>MNELVDTTEMYLRTIYDLEEEGVTPLRARIAERLDQSGPTVSQTVSRMERDGLLRVAGDRHLELTEKGRALAIAVMRKHRLAERLLVDVIGLPWEEVHAEACRWEHVMSEDVERRLVKVLNNPTTSPFGNPIPGLDELGVGPEPGADDANLVRLTELPAGSPVAVVVRQLTEHVQGDIDLITRLKDAGVVPNARVTVETTP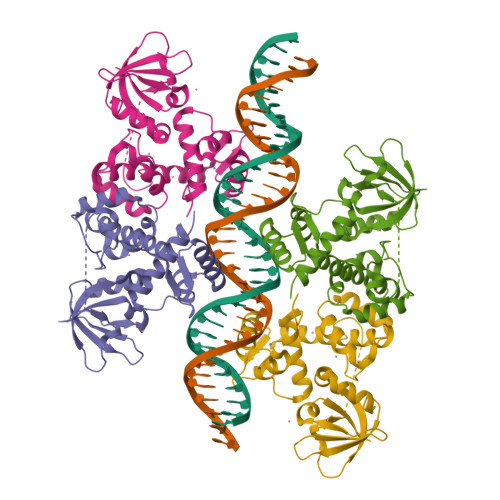GGGVTIVIPGHENVTLPHEMAHAVKVEKV[8x]> MSEFRIHHDVNELLSLLRVHGGDGAEVYIDLLQKNRTPYVTTTVSAHSAKVKIAEFSRTPEDFLKKYDELKSKNTRNLDPLVYLLSKLTEDKETLQYLQQNAKERAELAAAAVGSSTTSINVPAAASKISMQELEELRKQLGSVATGSTLQQSLELKRKMLRDKQNKKNSGQHLPIFPAWVYERPALIGDFLIGAGISTDTALPIGTLPLASQESAVVEDLLYVLVGVDGRYVSAQPLAGRQSRTFLVDPNLDLSIRELVHRILPVAASYSAVTRFIEEKSSFEYGQVNHALAAAMRTLVKEHLILVSQLEQLHRQGLLSLQKLWFYIQPAMRTMDILASLATSVDKGECLGGSTLSLLHDRSFSYTGDSQAQELCLYLTKAASAPYFEVLEKWIYRGIIHDPYSEFMVEEHELRKERIQEDYNDKYWDQRYTIVQQQIPSFLQKMADKILSTGKYLNVVRECGHDVTCPVAKEIIYTLKERAYVEQIEKAFNYASKVLLDFLMEEKELVAHLRSIKRYFLMDQGDFFVHFMDLAEEELRKPVEDITPPRLEALLELALRMSTANTDPFKDDLKIDLMPHDLITQLLRVLAIETKQEKAMAHADPTELALSGLEAFSFDYIVKWPLSLIINRKALTRYQMLFRHMFYCKHVERQLCSVWISNKTAKQHSLHSAQWFAGAFTLRQRMLNFVQNIQYYMMFEVMEPTWHILEKNLKSASNIDDVLGHHTGFLDTCLKDCMLTNPELLKVFSKLMSVCVMFTNCMQKFTQSMKLDGELGGQTLEHSTVLGLPAGAEERARKELARKHLAEHADTVQLVSGFEATINKFDKNFSAHLLDLLARLSIYSTSDCEHGMASVISRLDFNGFYTERLERLSAERSQKATPQVPVLRGPPAPAPRVAVTAQ;>[2x]MATPDQKSPNVLLQNLCCRILGRSEADVAQQFQYAVRVIGSNFAPTVERDEFLVAEKIKKELIRQRREADAALFSELHRKLHSQGVLKNKWSILYLLLSLSEDPRRQPSKVSSYATLFAQALPRDAHSTPYYYARPQTLPLSYQDRSAQSAQSSGSVGSSGISSIGLCALSGPAPAPQSLLPGQSNQAPGVGDCLRQQLGSRLAWTLTANQPSSQATTSKGVPSAVSRNMTRSRREGDTGGTMEITEAALVRDILYVFQGIDGKNIKMNNTENCYKVEGKANLSRSLRDTAVRLSELGWLHNKIRRYTDQRSLDRSFGLVGQSFCAALHQELREYYRLLSVLHSQLQLEDDQGVNLGLESSLTLRRLLVWTYDPKIRLKTLAALVDHCQGRKGGELASAVHAYTKTGDPYMRSLVQHILSLVSHPVLSFLYRWIYDGELEDTYHEFFVASDPTVKTDRLWHDKYTLRKSMIPSFMTMDQSRKVLLIGKSINFLHQVCHDQTPTTKMIAVTKSAESPQDAADLFTDLENAFQGKIDAAYFETSKYLLDVLNKKYSLLDHMQAMRRYLLLGQGDFIRHLMDLLKPELVRPATTLYQHNLTGILETAVRATNAQFDSPEILRRLDVRLLEVSPGDTGWDVFSLDYHVDGPIATVFTRECMSHYLRVFNFLWRAKRMEYILTDIRKGHMCNAKLLRNMPEFSGVLHQCHILASEMVHFIHQMQYYITFEVLECSWDELWNKVQQAQDLDHIIAAHEVFLDTIISRCLLDSDSRALLNQLRAVFDQIIELQNAQDAIYRAALEELQRRLQFEEKKKQREIEGQWGVTAAEEEEENKRIGEFKESIPKMCSQLRILTHFYQGIVQQFLVLLTTSSDESLRFLSFRLDFNEHYKAREPRLRVSLGTRGRRSSHT;>MIHELLLALSGYPGSIFTWNKRSGLQVSQDFPFLHPSETSVLNRLCRLGTDYIRFTEFIEQYTGHVQQQDHHPSQQGQGGLHGIYLRAFCTGLDSVLQPYRQALLDLEQEFLGDPHLSISHVNYFLDQFQLLFPSVMVVVEQIKSQKIHGCQILETVYKHSCGGLPPVRSALEKILAVCHGVMYKQLSAWMLHGLLLDQHEEFFIKQGPSSGNVSAQPEEDEEDLGIGGLTGKQLRELQDLRLIEEENMLAPSLKQFSLRVEILPSYIPVRVAEKILFVGESVQMFENQNVNLTRKGSILKNQEDTFAAELHRLKQQPLFSLVDFEQVVDRIRSTVAEHLWKLMVEESDLLGQLKIIKDFYLLGRGELFQAFIDTAQHMLKTPPTAVTEHDVNVAFQQSAHKVLLDDDNLLPLLHLTIEYHGKEHKADATQAREGPSRETSPREAPASGWAALGLSYKVQWPLHILFTPAVLEKYNVVFKYLLSVRRVQAELQHCWALQMQRKHLKSNQTDAIKWRLRNHMAFLVDNLQYYLQVDVLESQFSQLLHQINSTRDFESIRLAHDHFLSNLLAQSFILLKPVFHCLNEILDLCHSFCSLVSQNLGPLDERGAAQLSILVKGFSRQSSLLFKILSSVRNHQINSDLAQLLLRLDYNKYYTQAGGTLGSFGM[2x];>[2x]MARHGPPWSRLDAQQERDVRELVRGVAGLQDEADPNFQLALNFAWSNFRFHRFLDVNSHKIEKTIEGIYEKFVIHSDLSKAASWKRLTEEFLNAPLPSIKEIKTDAHYSILSLLLCLSDSPSNSSYVETPRNKEVEKKDDFDWGKYLMEDEEMDIGPYMDTPNWSEESEEENDQQPLSREDSGIQVDRTPLEEQDQNRKLDPCISWKDEPDDRSWLEHHVVHQYWTARPSQFPHSLHLHSNLAAVWDQHLYSSDPLYVPDDRVLVTETQVIRETLWLLSGVKKLFIFQLIDGKVTVRNNIIVTHLTHSCLRSVLEQIAAYGQVVFRLQEFIDEVMGHSSESMLPGSGSVPKKSTEAPFRTYQAFMWALYKYFISFKEELAEIEKCIINNDTTITLAIVVDKLAPRLSQLKVLHKVFSTGVAEVPPDTRNVVRASHLLNTLYKAILEYDNVGEASEQTVSLLFSLWVETVRPYLQTVDEWIVHGHLWDGAREFIIQRNKNVPVNHRDFWYATYTLYSVSEKTENEEKMSDNASASSGSDQGPSSRQHTMVSFLKPVLKQIIMAGKSMQLLKNLQCAESTTCQAGARDAERKSLYTLFLESVQSRLRHGEDSTPQVLTEQQATKENLMKMQSIAESHLELDDVHDPLLAINFARMYLEQSDFHEKFAGGDVCVDRSSESVTCQTFELTLRSCLYPHIDKQYLDCCGNLMQTLKKDYRLVEYLQAMRNFFLMEGGDTMYDFYTSIFDKIREKETWQNVSFLNVQLQEAVGQRYPEDSSRLSISFENVDTAKKKLPVHILDGLTLSYKVPWPVDIVISLECQKIYNQVFLLLLQIKWAKYSLDVLLFGELVSTAEKPRLKEGLIHEQDTVAQFGPQKEPVRQQIHRMFLLRVKLMHFVNSLHNYIMTRILHSTGLEFQHQVEEAKDLDQLIKIHYRYLSTIHDRCLLREKVSFVKEAIMKVLNLALMFADGWQAGLGTWRMESIEKMESDFKNCHMFLVTILNKAVCRGSFPHLESLALSLMAGMEQS;> MASITQLFDDLCEALLPAAKTHLGQRSVNRKRAKRSLKKVAYNALFTNLFQDETQQLQPDMSKLPARNKILMLSFDLRVGGLGPKADRLEELVEELEAAPCCPLLEVGSVLDLLVQLAGSGPPQVLPRKRDYFLNNKHVGRNVPYSGYDCDDLSVFEMDVQSLISREECLCHSMIQETLQVMEAAPGTGLPTVGLFSFGDPCGDRFERDTRVSLFGALVHSRTYDMDVRLGLPPVPDNADLSGLAIKVPPSVDQWEDEGFQSASNLTPDSQSEPSVTPDVDLWEAALTYEASKRRCWERVGCPPGHREEPYLTEAGRDAFDKFCRLHQGELQLLAGGVLQAPQPVLVKECELVKDVLNVLIGVVSATFSLCQPAQAFVVKRGVHVSGASPESISSLLSEVAEYGTCYTRLSHFSLQPVLDSLYSKGLVFQAFTSGLRRYLQYYRACVLSTPPTLSLLTIGFLFKKLGRQLRYLAELCGVGAVLPGTCGGGPRAAFPTGVKLLSYLYQEALHNCSNEHYPVLLSLLKTSCEPYTRFIHDWVYSGVFRDAYGEFMIQVNHEYLSFRDKLYWTHGYVLISKEVEDCVPVFLKHIAHDIYVCGKTINLLKLCCPRHYLCWSDVPVPRISVIFSLEELKEIEKDCAVYVGRMERVARHSSVSKEEKELRMEIAKQELIAHAREAASRVLSALSDRQMSERMALDARKREQFQRLKEQFVKDQERRQAARQEELDDDFSYARELRDRERRLKSLEEELERKARQALVDHYSKLSAEAARREQKALWRIQRHRLESARLRFLLEDEKHIQEMLKAVSEAHQPQEPPDVLLSVHPQVTSPGPEHPEGGQGCDSGSAEQHSPAWDGWNRPGLLTPQPLKPLAVGAGGRGLQQAEGARPFSDSLSIGDFLPVGPGAEPSVQTGMVPLLEVALQTINLDLPPSAPGEAPAAASTQPSRPQEYDFSTVLRPAVATSPAPGPLQAAECSLGSSGLQLWEDSCGKMDACGSASRETLLPSHPPRRAALEEGSSQPTERLFGQVSGGGLPTGDYASEIAPTRPRWNTHGHVSDASIRVGENVSDVAPTQPRWNTHGHVSNASISLGESVSDVAPTRPRWNIHGHVSNASIRVGENVSDVAPTRPRWNTHGHVSNASIRVGENVSDVAPTRPRWNTHGHVSDASISLGESVSDMAPARPRWNTHGHVSDASISLGESVSDMAPTRPRWNTHGHVSDTSIRVGENVSDVAPIRSRCNTHGHVSDASISLGEPVSDVVSTRPRWNTHVPIPPPHMVLGALSPEAEPNTPRPQQSPPGHTSQSALSLGAQSTVLDCGPRLPVEVGPSLSSPSSGCGEGSISVGENVSDVAPTQPWWPNTPGDSVSEELGPGRSGDTEDLSPNWPLNSQEDTAAQSSPGRGEEAEASAAEAQGGEQAYLAGLAGQYHLERYPDSYESMSEPPIAHLLRPVLPRAFAFPVDPQVQSAADETAVQLSELLTLPVLMKRSITAPLAAHISLVNKAAVDYFFVELHLEAHYEALRHFLLMEDGEFAQSLSDLLFEKLGAGQTPGELLNPLVLNSVLSKALQCSLHGDTPHASNLSLALKYLPEVFAPNAPDVLSCLELRYKVDWPLNIVITEGCVSKYSGVFSFLLQLKLMMWALKDVCFHLKRTALLSHMAGSVQFRQLQLFKHEMQHFVKVIQGYIANQILHVTWCEFRARLATVGDLEEIQRAHAEYLHKAVFRGLLTEKAAPVMNVIHSIFSLVLKFRSQLISQAWGPPGGPRGAEHPNFALMQQSYNTFKYYSHFLFKVVTKLVNRGYQPHLEDFLLRINFNNYYQDA;>[6x]MPREIITLQLGQCGNQIGFEFWKQLCAEHGISPEGIVEEFATEGTDRKDVFFYQADDEHYIPRAVLLDLEPRVIHSILNSPYAKLYNPENIYLSEHGGGAGNNWASGFSQGEKIHEDIFDIIDREADGSDSLEGFVLCHSIAGGTGSGLGSYLLERLNDRYPKKLVQTYSVFPNQDEMSDVVVQPYNSLLTLKRLTQNADCVVVLDNTALNRIATDRLHIQNPSFSQINQLVSTIMSASTTTLRYPGYMNNDLIGLIASLIPTPRLHFLMTGYTPLTTDQSVASVRKTTVLDVMRRLLQPKNVMVSTGRDRQTNHCYIAILNIIQGEVDPTQVHKSLQRIRERKLANFIPWGPASIQVALSRKSPYLPSAHRVSGLMMANHTSISSLFERTCRQYDKLRKREAFLEQFRKEDMFKDNFDEMDTSREIVQQLIDEYHAATRPDYISWGTQEQ;>[2x]MASSSGAGAAAAAAAANLNAVRETMDVLLEISRILNTGLDMETLSICVRLCEQGINPEALSSVIKELRKATEALKAAENMTS

The gamma-tubulin ring complex (γ-TuRC) is the principal microtubule nucleation template in vertebrates. Microtubules are formed de novo in a process termed nucleation, which is spatially and temporally highly controlled by γ-tubulin complexes, composed of γ-tubulin1 and associated γ-tubulin-complex proteins (GCP). In most eukaryotes, microtubules are templated from a preassembled γ-tubulin ring complex (γ-TuRC) that determines the position and direction of microtubule growth. Here, we used cryo-EM to identify and characterize γ-TuRC assembly intermediates after recombinant expression of the complex, which allowed us to delineate a comprehensive stepwise assembly pathway from a stable 6-spoked core to the mature 14-spoked γ-TuRC, identifying successive stabilization and conformational locking of γ-TuSC units as central principles in the assembly process.

Extensive 3D classification revealed a core of six γ-tubulin-GCP spokes as the minimal stable and most abundant entity in this experiment. This 6-spoke assembly intermediate was resolved to 5.3 Å resolution, sufficient to unambiguously determine the identity and sequential arrangement of spokes based on secondary structure features of the GCP proteins. The cryo-EM density of the 6-spoke intermediate revealed that the first module of the lumenal bridge has already been formed by recruitment of the MZT1-GCP3 module to the GCP3(8) GRIP1 domain. Since only one copy of GCP3 is present in this intermediate, this clearly indicates that the MZT1-GCP3 module of GCP3(8) (rather than any other copy of GCP3) is involved in forming the lumenal bridge. Surprisingly, the outer surface of the GCP3(8) GRIP2 domain is associated with an additional MZT1-containing module. As the only MZT1-GCP3 module present in the 6-spoke intermediate was already stably recruited into the lumenal bridge, MZT1-GCP5 and MZT1-GCP6 were the only other candidates to represent this additional MZT1 module. Notably, GCP3(8) and the adjacent GCP4(9) subunit create a structurally unique binding site for this MZT1-GCP5 module, which likely explains the specific binding of MZT1-GCP5 to the outer surface of GCP3(8), while MZT1-GCP3(8) remains available to form the first module of the lumenal bridge. The overall stabilizing role of the GCP6 GRIP1-NTE is further supported by direct contacts of GCP6 with the GCP5(10) GRIP1-NTE and the GRIP1 domains of GCP4(9), GCP5(10), and GCP4(11), effectively bridging all GCP subunits of the intermediate. Taken together, we conclude that the GCP6 GRIP1-NTE plays a central role in the formation of the stable 6-spoke intermediate, providing a structure-based rationale for the effects of GCP6 truncations on γ-TuRC assembly previously observed in sucrose gradient sedimentation experiments.> MNGDETKKVESEYIKKHHRHELVESQCSSTLVKHIKAPL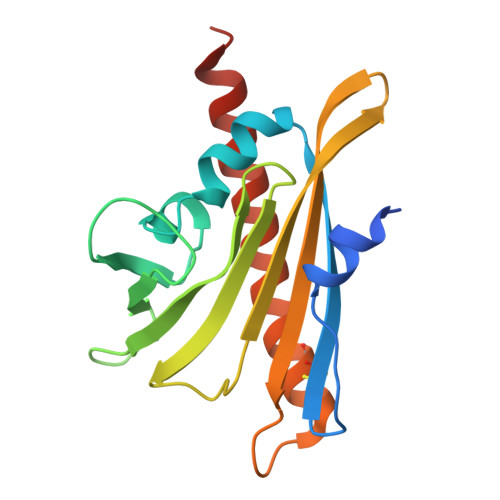HLVWSIVRRFDEPQKYKPFISRCVVQGKKLEVGSVREVDLKSGLPATKSTEVLEILDDNEHILGIRIVGGDHRLKNYSSTISLHSETIDGKTGTLAIESFVVDVPEGNTKEETCFFVEALIQCNLNSLADVTERLQAESMEKKI>MGRDRRHKMETIEGVVVVGGGPVGLLTALKLGKAGVRVVVLESESGVSPSPRAVAYMPPTAAALDRFGLLDDIRKRAVWCPDFAYRHGNGELIAKMDWAVLAQDTDYPYMLLLAQNHVSNVIVEHLRKLPNVEIRWNHKVEEIDQDDDYVTMETSGPAGKASLRAKWVAATDGARSTVRGKIGLTFDGITWSERLVATNVFYDFSLHGYSRANFVHDPVDWAVVVQLDKTGLWRVCYGEDPDISEAEVRRRLPERFKRLLPGAPTPDQYRVDYLNPYRVHQRCAAEFRRGRVILAGDAAHATNPMGGLGLSGGVLDAEHLAEALIAVIKEGASTKVLDEYSVDRRKVFLEFTSPTATANFTWMKESDPAQRARDNAMFDHAGKDLKVMREILLDF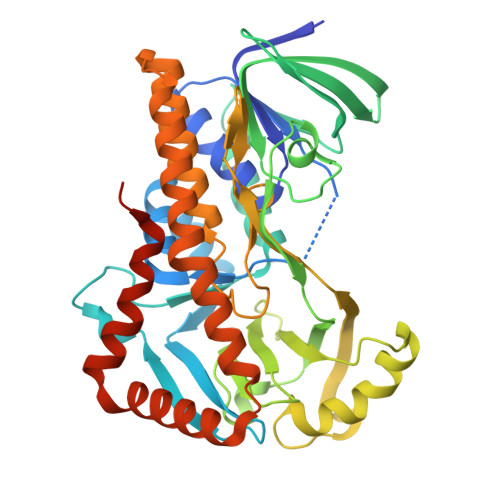EKLNGRRVIAPRQHAPEHELVGA[2x]> TIQPGTGYNNGYFYSYWNDGH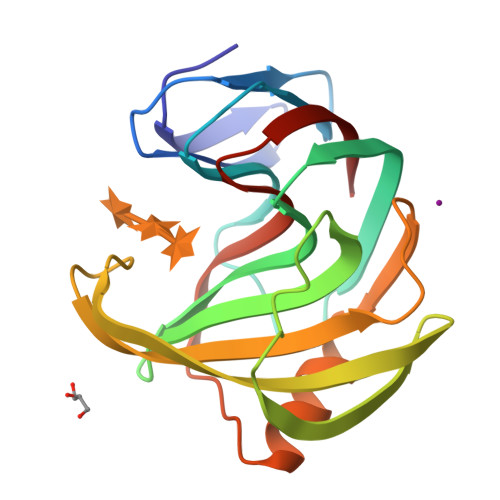GGVTYTNGPGGQFSVNWSNSGDFVGGKGWQPGTKNKVINFSGSYNPNGNSYLSVYGWSRNPLIEYYIVENFGTYNPSTGATKLGEVTSDGSVYDIYRTQRVNQPSIIGTATFYQYWSVRRNHRSSGSVNTANHFNAWAQQGLTLGTMDYQIVAVEGYFSSGSASITVS>[2x]MAAESVRVAVRCRPFNQREKDLNTTLCVGMTPNVGQVNLNAPDGAAKDFTFDGAYFMDSTGEQIYNDIVFPLVENVIEGYNGTVFAYGQTGSGKTFSMQGIETIPAQRGVIPRAFDHIFTATATTENVKFLVHCSYLEIYNEEVRDLLGADNKQKLEIKEQPDRGVYVAGLSMHVCHDVPACKELMTRGFNNRHVGATLMNKDSSRSHSIFTVYVEGMTETGSIRMGKLNL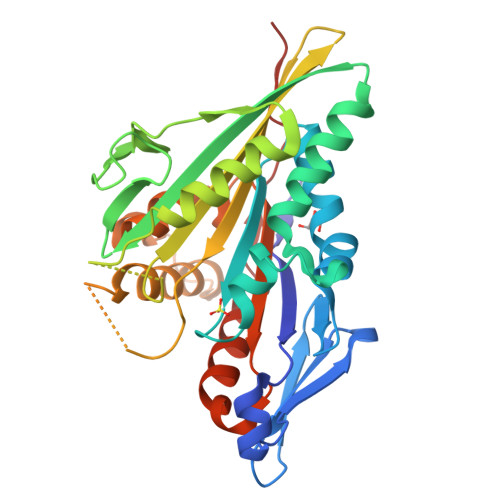VDLAGSERQSKTGATGDRLKEATKINLSLSALGNVISALVDGKSKHIPYRDSKLTRLLQDSLGGNTKTIMIACVSPSSDNYDETLSTLRYANRAKNIKNKPTINEDPLEHHHHHH>GSHMGGIEVLGVKTGVDSFTEVECFLNPQMGNPDEHQKGLSKSLAAEKQFTDDSPDKEQLPCYSVARIPLPNINEDLTCGNILMWEAVTVKTEVIGVTAMLNLHSGTQKTHENGAGKPIQGSNFHFFAVGGEPLELQGVLANYRTKYPAQTVTPKNATVDSQQMNTDHKAVLDKD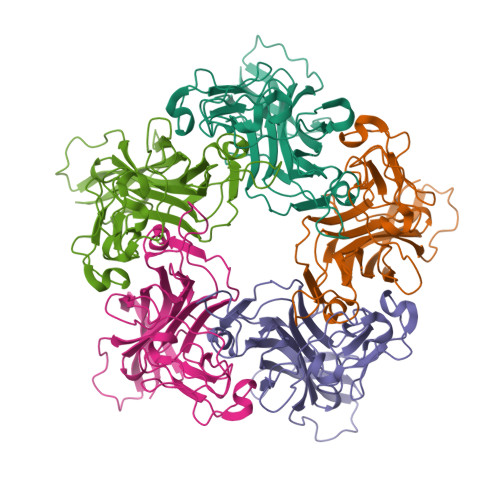NAYPVECWVPDPSKNENTRYFGTYTGGENVPPVLHITNTATTVLLDEQGVGPLCKADSLYVSAVDICGLFTNTSGTQQWKGLPRYFKITLRKRSVKN[5x]>[2x]GMSPPAPADVVSSAKPHVAVIPAAGMGHLNPTLRLAGELASRGCVVTFINPSPPVSLAEATSVAEFVASTPGVRLLDLPVQPLDPSCFPAHEDPFLRQFEAVRRSAPLLTPLLSDVSPPLAAIVCDIAICSTFLTVAAEISLPAYVFFSLSAQMLSLNLAFPTVADQVYGAGEGDEIRFPGLPESIPRSWLPPPLLDPAHLFAVHFVENGKAMPRAAG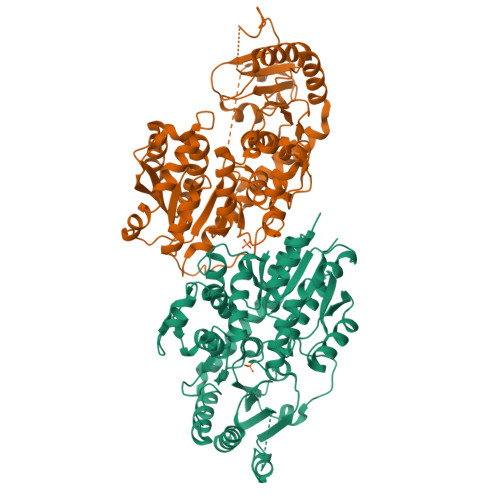ILVHSWEALEPEALAALRGGRVLAGLPPVLPIGPLYQKEKSNAVFLPWLDAQRDRSVLFVCFGNRSTHSPEQLREMAAGLERSGCRFVWVLKTKVVDKDEDEGAQKEILGEGYLERVKERGVVINGWVDQMTILSHRAVGGFFSHSGSSSVAEAAIGGQPLLLWPMGGDQRMSALVAERRGMGVWPRGWGWSADDKLIPGEEIARRIKDFMGDNALRAVAAKMKKETASAMAPGGSKDQWFDDFIARINRV> GPSSRRAKSVEDDAEGHLIYHVGDWLQERYEIVSTLGEGTFGRVVQCVDHRRGGARVALKIIKNVEKYKEAARLEINVLEKINEKDPDNKNLCVQMFDWFDYHGHMCISFELLGLSTFDFLKDNNYLPYPIHQVRHMAFQLCQAVKFLHDNKLTHTDLKPENILFVNSDYELTYNLEKKRDERSVKSTAVRVVDFGSATFDHEHHSTIVSTRHYRAPEVILELGWSQPCDVWSI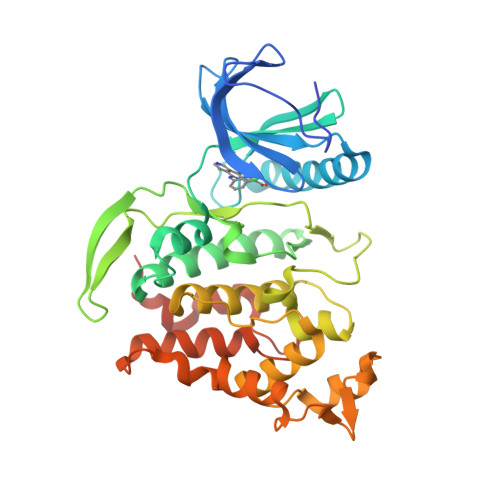GCIIFEYYVGFTLFQTHDNREHLAMMERILGPIPSRMIRKTRKQKYFYRGRLDWDENTSAGRYVRENCKPLRRYLTSEAEEHHQLFDLIESMLEYEPAKRLTLGEALQHPFFARLRAEPPNKLWDSSRD>GAMDEKFIRETIETRIMMEVFCLENYFDKIAGSEELLEIKGEIDDVAASAAREIFDDSDERLHKLFIRASGNELIISLYEKIWDRIDLVRHLNERYVVSNREHKELIERIISGDKE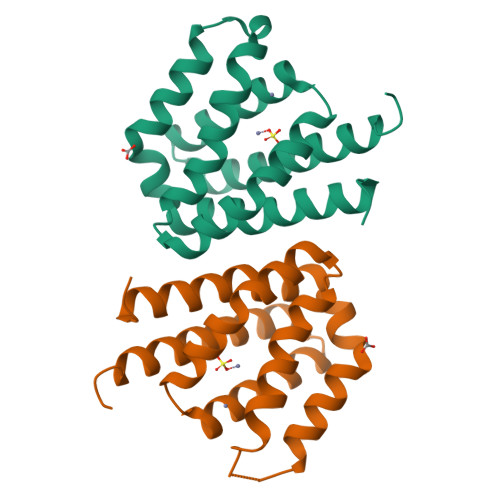GAIEKLKEHLKNVEAETIKNLYTY[2x]>[2x]EVKLILYHWTHSFSSQKVRLVIAEKALKCEEHDVSLPLSEHNEPWFMRLNSTGEVPVLIHGE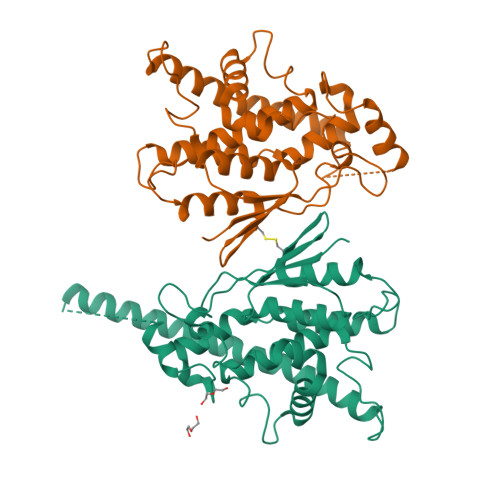NIICEATQIIDYLEQTFLDERTPRLMPDKESMYYPRVQRYRELLDSLPMDAYTHGCILHPELTVDSMIPAYATTRIRSQIGNTESELKKLAEENPDLQEAYIAKQKRLKSKLLDHDNVKYLKKILDELEKVLDQVETELQRRNEETPEEGQQPWLCGESFTLADVSLAVTLHRLKFLGFARRNWGNGKRPNLETYYERVLKRKTFNKVLGHVNNILIS Lipopolysaccharides such as the enterobacterial common antigen are important components of the enterobacterial cell envelope that act as a protective barrier against the environment and are often polymerized by the inner membrane bound Wzy-dependent pathway. By employing cryo-electron microscopy we show that WzzE, the co-polymerase component of this pathway that is responsible for the length modulation of the enterobacterial common antigen, is octameric with alternating up-down conformations of its L4 loops. The alternating up-down nature of these essential loops, located at the top of the periplasmic bell, are modulated by clashing helical faces between adjacent protomers that flank the L4 loops around the octameric periplasmic bell. This alternating arrangement and a highly negatively charged binding face create a dynamic environment in which the polysaccharide chain is extended, and suggest a ratchet-type mechanism for polysaccharide elongation.

We purified and determined the structure of the fully intact polysaccharide co-polymerase WzzE from E. coli by cryo-electron microscopy to an overall resolution of 3.2 Å. An overall resolution of 3.4 Å was obtained without the application of symmetry and, although clearly octameric in nature, displayed a loss of octameric symmetry in the region of the L4 loops at the top of the periplasmic bell. In this region the L4 loops are seen in two conformations, one up and one down with, remarkably, the subunits clearly alternating between the up and down conformations around the octameric complex. Although the application of C8 symmetry did marginally improve the overall resolution of the map to 3.1 Å, the alternating nature of the L4 region was averaged out. Thus, in order to resolve this alternating arrangement of loops, C4 symmetry was applied by using two adjacent subunits encompassing the two L4 conformations as the asymmetric unit resulting in a 3.2 Å map. The high quality of the C4 symmetrized map allowed the complete amino acid sequence of the periplasmic domain to be built, including the dynamic L4 loops in alternating conformations. Within WzzE, this alternating arrangement of the L4 loops results in a subtle rearrangement of its two flanking helices (α6 and α7): when in the upward facing position α6 helix is tilted approximated 9° outwards away from α7, and is slightly elongated suggesting that a slight unraveling occurs when L4 is in the downward position; and when the L4 loop is in the downward position α7 tilts slightly inwards towards the center of the periplasmic bell. Thus, as a consequence of the up-down nature of the L4 loops the full octameric structure of WzzE contains a 13 Å opening at the top of its periplasmic bell nearly double the distance compared to that of WzzB containing all downward L4 loops at 7.5 Å at their narrowest points.

>[8x]MTQPMPGKPAEDAENELDIRGLFRTLWAGKLWIIGMGLAFALIALAYTFFARQEWSSTAITDRPTVNMLGGYYSQQQFLRNLDVRSNMASADQPSVMDEAYKEFVMQLASWDTRREFWLQTDYYKQRMVGNSKADAALLDEMINNIQFIPGDFTRAVNDSVKLIAETAPDANNLLRQYVAFASQRAASHLNDELKGAWAARTIQMKAQVKRQEEVAKAIYDRRMNSIEQALKIAEQHNISRSATDVPAEELPDSEMFLLGRPMLQARLENLQAVGPAFDLDYDQNRAMLNTLNVGPTLDPRFQTYRYLRTPEEPVKRDSPRRAFLMIMWGIVGGLIGAGVALTRRCSKEFRVPGSHHHHHHHH> Y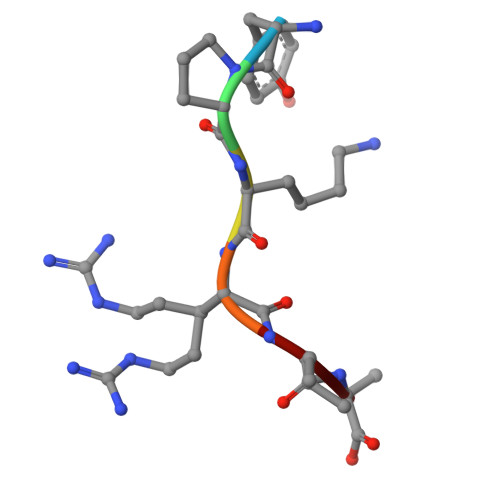PKRIA>[4x]LEEKKVC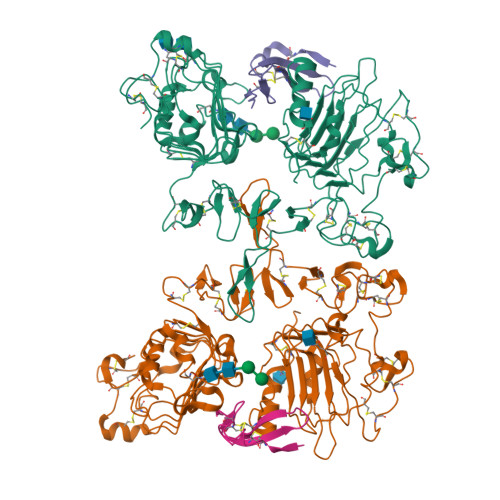QGTSNKLTQLGTFEDHFLSLQRMFNNCEVVLGNLEITYVQRNYDLSFLKTIQEVAGYVLIALNTVERIPLENLQIIRGNMYYENSYALAVLSNYDANKTGLKELPMRNLQEILHGAVRFSNNPALCNVESIQWRDIVSSDFLSNMSMDFQNHLGSCQKCDPSCPNGSCWGAGEENCQKLTKIICAQQCSGRCRGKSPSDCCHNQCAAGCTGPRESDCLVCRKFRDEATCKDTCPPLMLYNPTTYQMDVNPEGKYSFGATCVKKCPRNYVVTDHGSCVRACGADSYEMEEDGVRKCKKCEGPCRKVCNGIGIGEFKDSLSINATNIKHFKNCTSISGDLHILPVAFRGDSFTHTPPLDPQELDILKTVKEITGFLLIQAWPENRTDLHAFENLEIIRGRTKQHGQFSLAVVSLNITSLGLRSLKEISDGDVIISGNKNLCYANTINWKKLFGTSGQKTKIISNRGENSCKATGQVCHALCSPEGCWGPEPRDCVSHHHHHH;>SDNPRVAQVSITKCSSDMNGYCLHGQCIYLVDMSQNYCRCEVGYTGVRCEHFFLTVHQPLSK[4x]>MKIVLVLYDAGKHAADEEKLYGCTENKLGIANWLKDQGHELITTSDKEGGNSVLDQHIPDADIIITTPFHPAYITKERIDKAKKLKLVVVAGVGSDHIDLDYINQTGKKISVLEVTGSNTVSVAEHVLMTMLVLVRNFVPAHEQIINHDWEVAAIAKDAYDIEGKTIATIGAGRIGYRVLERLVPFNPKELLYYDYQALPKDAEEKVGARRVENIEELVAQADIVTINAPLHAGTKGLINKELLSKFKKGAWLVNTARGAICVAEDVAAALESGQLRGY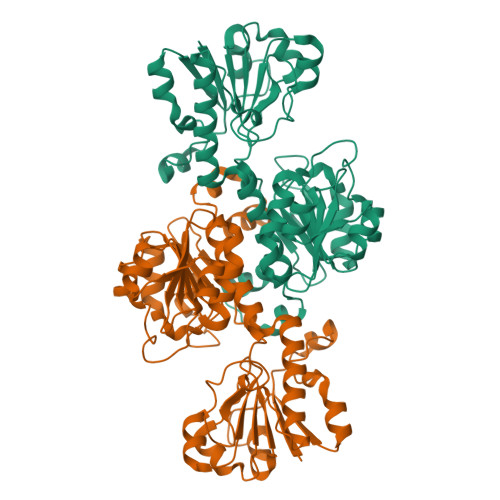GGDVWFPQPAPKDHPWRDMRNKYGAGNAMTPHYSGTTLDAQTRYAEGTKNILESFFTGKFDYRPQDIILLNGEYITKAYGKHDKK[4x]>QGPLGSKLSEHLRYCDSILREMLSKKHAAYAWPFYKPVDAEALELHDYHDIIKHPMDLSTVKRKMDGREYPDAQGFAADVRLMFSNCYKYNPPDHEVVAMARKLQDVFEMRFAKMPDEP[2x];> XWKQWKKYGLKICX

Within this class of proteins, the bromodomain and extraterminal domain (BET) family contains four members that are transcriptional coregulators and that recognize acetyllysines (AcKs) using a tandem pair of highly homologous bromodomains (BDs). Despite heavy academic and industry investment in this area, the generation of paralog-selective inhibitors has proved elusive because of the extremely high sequence similarity between the bromodomains of family members (90 to 95% within the acetyllysine-binding pocket residues). Using the highly conserved BET BDs as a model system, we conducted three mRNA display-based RaPID (random nonstandard peptides integrated discovery) screens using a single library (which contains >1012 unique members). Crystal structures of 13 distinct peptide–bromodomain complexes revealed highly diverse structures and binding modes among the cyclic peptide ligands.

Likewise, the most abundant family identified in the BRD3-BD2 selection (BRD3-BD2 family 3, accounting for 53% of total sequencing reads recovered for the top 500 peptides, including 3.2C) was not found in the BRD3-BD1 screen. In contrast, 3.2C bound to the BD2 domains with affinities of 10 to 100 nM but did not bind strongly to any BD1 domain, consistent with selectivities of >10- to 100-fold between these domains. Like 3.1B, both peptides bind two copies of the BD. In contrast to 3.1B, however, almost no direct contacts were observed between the two BDs, suggesting that in these cases crystallization might have promoted the bivalent interaction. The two AcK residues (AcK2 and AcK6) in the peptide each engage a BD via the AcK pocket although, in both cases, the N-acetyl moiety lies too far from the conserved Asn (Asn391) to form a direct hydrogen bond. It is likely that water-mediated interactions are formed, but the relatively low resolution of this structure (2.8 Å) prevented us from directly observing solvent water. The two peptide–BD interfaces bury 1,120 Å2 (BRD3-BD2-A) and 1,116 Å2 (BRD3-BD2-B) of surface area and the peptide contacts very similar surfaces in the two domains —a surface that significantly overlaps with the contact surface for 3.1C.> MASMTGGQQMGRIPGNSPRMVLLESEQFLTELTRLFQKCRSSGSVFITLKKYDGRTKPIPRKSSVEGLEPAENKCLLRATDGKRKISTVVSSKEVNKFQMAYSNLLRANMDGLKKRDKKNKSKKSKPAQGGEQKLISEEDDSAGSPMPQFQTWEEFSRAAEKLYLADPMKVRVVLKYRHVDGNLCIKVTDDLVCLVYRTDQAQDVKKIEKF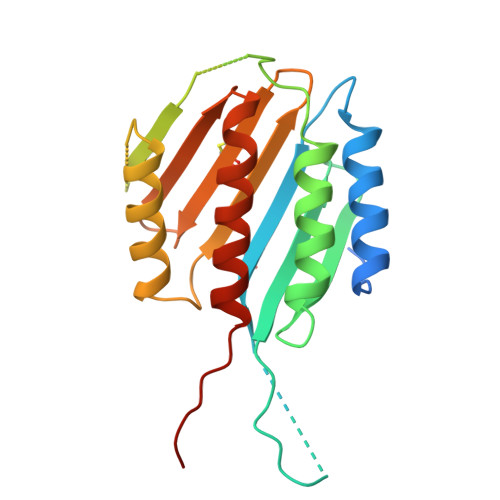HSQLMRLMVAKESRNVTMETE>MGHHHHHHVSSTNGFSATRSTVIQLLNNISTKREVEQYLKYFTSVSQQQFAVIKVGGAIISDNLHELASCLAFLYHVGLYPIVLHGTGPQVNGRLEAQGIEPDYIDGIRITDEHTMAVVRKCFLEQNLKLVTALEQLGVRARPITSGVFTADYLDKDKYKLVGNIKSVTKEPIEASIKAGALPILTSLAETASGQMLNVNADVAAGELARVFEPLKIVYLNEKGGIINGSTGEKISMINLDEEYDDLMKQSWVKYGTKLKIREIKELLDYLPRSSSVAIINVQDLQKELFTDSGAGTMIRRGYKLVK[4x]

The first step of the route is the production of N-acetyl-L-glutamate (NAG), while the second is the phosphorylation of NAG by NAG kinase (NAGK). We report here structural and functional studies on the arginine-sensitive NAGK from Saccharomyces cerevisiae (yNAGK). The structure of the mature yNAGK, lacking the N-terminal mitochondrial targeting sequence (residues 1–57), reveals an unexpected novel tetrameric architecture, which can be described as a dimer of dimers with D2 symmetry. The AAK domains occupy the center of the molecule flanked by two pairs of interacting DUF619 domains.

A truncated form of yNAGK spanning from residue 58 to 356, corresponding to the AAK domain and lacking the C-terminal DUF619 domain, was produced as a soluble protein in milligram amounts in E. coli. Four crystal structures of truncated yNAGK, ligand-free or complexed with either NAG or NAG and arginine, were determined using for the initial phasing single anomalous diffraction (SAD) from a Se-Met derivative. Four subunits, organized as a dimer of dimers with D2 local symmetry, were found in the asymmetric unit of these crystals. In the crystals containing NAG, one NAG molecule was found in each subunit. As reported in other NAGKs (best studied in EcNAGK), NAG is bound in a pocket in the N-lobe under the closed lid formed by the β3–β4 hairpin. Despite the different oligomerization of yNAGK in relation to other NAGKs, the AAK domain structure closely conforms to the canonic α3β8α4 sandwich NAGK subunit fold, with the N-lobe spanning residues 96–272 and the C-lobe residues 273–350. In yNAGK, the β5 strands of the two subunits still interact with each other, although they are parallel due to the large rotation of one subunit relative to the other. At each interdimeric junction, a four-helix bundle is formed by both interacting “stands”, burying an approximate area of 910 Å2 per subunit. In any case, the interactions mediated by these stands result in the association of two yNAGK dimers into a relatively flat rectangular tetramer with approximate dimensions of 35 Å×109 Å×83 Å. Two active centers, separated by a distance of 80 Å, are exposed in one diagonal on each face of the tetramer.> TWLSDFPQAWAETGGMGLAVRQAPLIIPLKATSTPVSIKQYPMSQEARLGIKPHIQRLLDQGILVPCQSPWNTPLLPV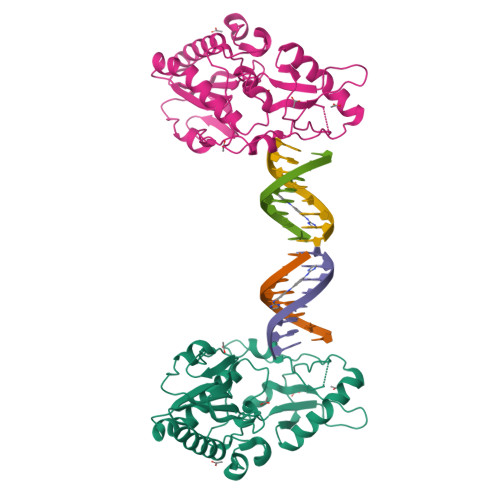KKPGTNDYRPVQDLREVNKRVEDIHPTVPNPYNLLSGLPPSHQWYTVLDLKDAFFCLRLHPTSQPLFAFEWRDPEMGISGQLTWTRLPQGFKNSPTLFDEALHRDLADFRIQHPDLILLQYVDDLLLAATSELDCQQGTRALLQTLGNLGYRASAKKAQICQKQVKYLGYLLKEGQR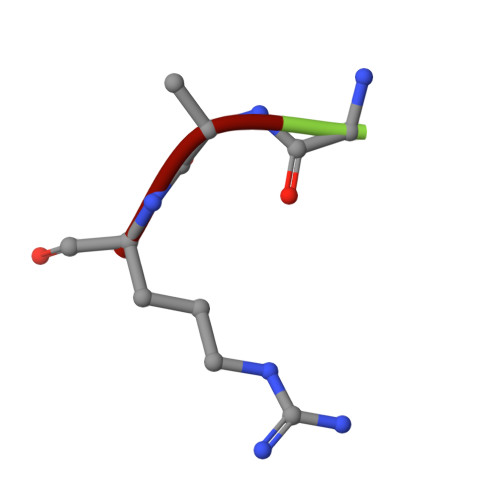> GAR>SGIDEEELIEAADFQGLYAEVKACSSELESLEMELRQQILVNIGKILQDQPSMEALEASLGQGLCSGGQVEPLDGPAGCILECLVLD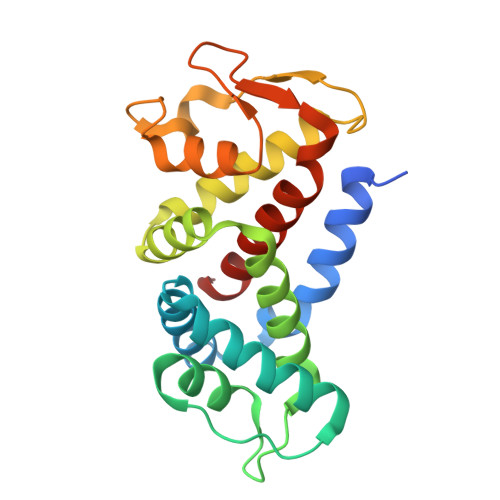SGELVPELAAPIFYLLGALAVLSETQQQLLAKALETTVLSKQLELVKHVLEQSTPWQEQSSVSLPTVLLGDCWDEKNPTWVLLEECGLRLQVESPQVHWEPTSLIPTSALYASLFLLSSLGQKPC[4x]> KDGDQCETSPCQNQGKCKDGLGEYTCTCLEGFEGKNCELFTRKLCSLDNGDCDQFCHEEQNSVVCSCARGYTLAD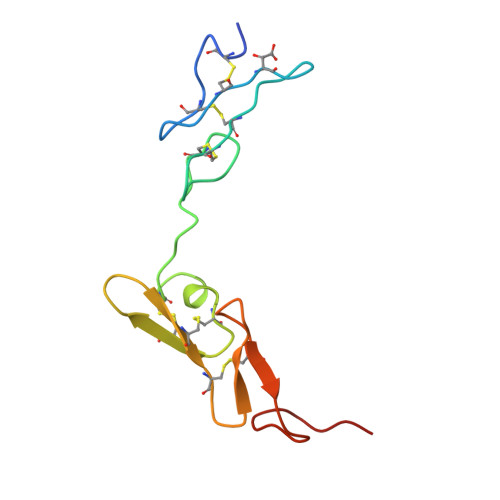NGKACIPTGPYPCGKQTLER> MKTINLSIFGLGNVGLNLLRIIRSFNEENRLGLKFNVVFVADSLHSYYNERIDIGKVISYKEKGSLDSLEYESISASEALARDFDIVVDATPASADGKKELAFYKETFENGKDVVTANKSGLANFWPEIMEYARSNNRRIRYEATVAGGVPLFSFIDYSVLPSRIKKFRGIVSLTINYFIRELANKREFDDVLSEATKLGIVEKNYKDDLTGLDAARKSVILCNHLYGSSYRL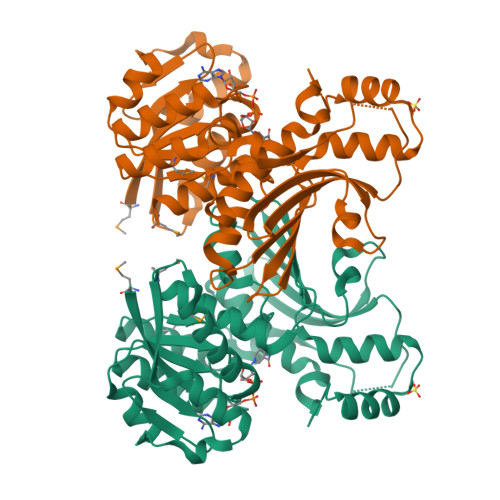SDVFYEGILDQDRSFGKNERLVTETGIVNGKPSAESRIKSLDSNDYLLTLGKGSLGYQLQTDTNGTLNVSDLYDGPYETAGAVMNDLVILSMFTV> EKSVVFKAEGEHFTDQKGNTIVGSGSGGTTKYFRIPAMCTTSKGTIVVFADARHNTASGQSFIDTAAARSTDGGKTWNKKIAIYNDRVNSKLSRVMDPTCIVANIQGRETILVMVGKWNNNDKTWGAYRDKAPDTDWDLVLYKSTDDGVTFSKVETNIHDIVTKNGTISAMLGGVGSGLQLNDGKLVFPVQMVRTKNITTVLNTSFIYSTDGITWSLPSGYCEGFGSENNIIEFNASLVNNIRNSGLRRSFETKDFGKTWTEFPPMDKKVDNRNHGVQGSTITIPSGNKLVAAHSSAQNKNNDYTRSDISLYAHNLYSGEVKLIDDFYPKVGNASGAGYSCLSYRKN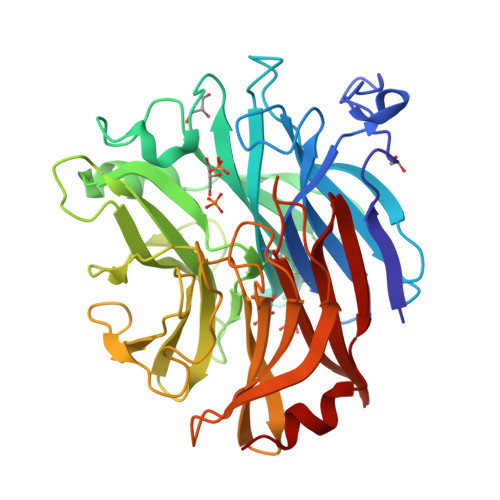VDKETLYVVYEANGSIEFQDLSRHLPVIKSYN> SHGLSFSPPLSVADGVVSLDMDPYFCSQRVSLTSYSAEAQLMQFRWMARGTNGSSDTIDMTVNAHCHGRRTDYMMSSTGNLTV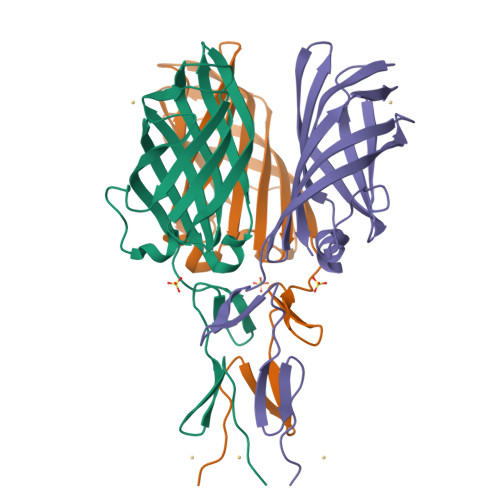TSNVVLLTFDLSDITHIPSDLARLVPSAGFQAASFPVDVSFTRDSATHAYQAYGVYSSSRVFTITFPTGGDGTANIRSLTVRTGIDT> MEEPEEPADSGQSLVPVYIYSPEYVSMCDSLAKIPKRASMVHSLIEAYALHKQMRIVKPKVASMEEMATFHTDAYLQHLQKVSQEGDDDHPDSIEYGLGYDCPATEGIFDYAAAIGGATITAAQCLIDGMCKVAINWSGGWHHAKKDEASGF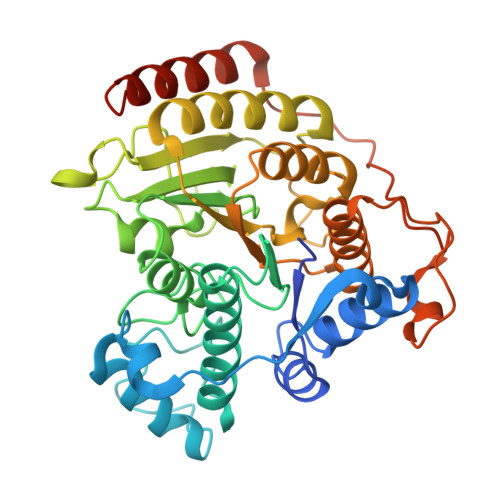CYLNDAVLGILRLRRKFERILYVDLDLHHGDGVEDAFSFTSKVMTVSLHKFSPGFFPGTGDVSDVGLGKGRYYSVNVPIQGGIQDEKYYQICESVLKEVYQAFNPKAVVLQLGADTIAGDPMCSFNMTPVGIGKCLKYILQWQLATLILGGGGFNLANTARCWTYLTGVILGKTLSSEIPDHEFFTAYGPDYVLEITPSCRPDRNEPHRIQQILNYIKGNLKHVVIEGRGSHHHHHH>[2x]GPMKTEMKDDFAKLEEQFDAKLGIFALDTGTNRTVAYRPDERFAFASTIKALTVGVLLQQKSIEDLNQRITYTRDDLVNYNPITEKHVDTGMTLKELADASLRYSDNAAQNLILKQIGGPESLKKELRKIG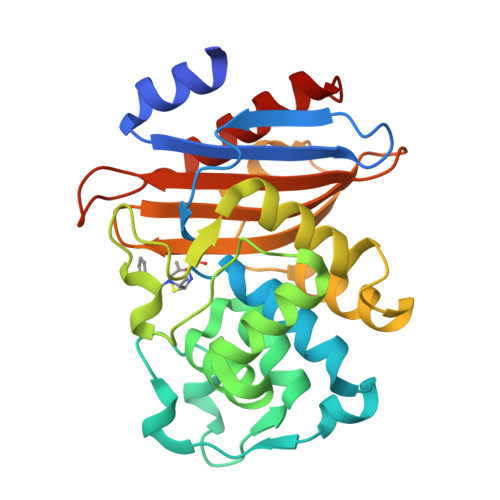DEVTNPERFYPELNEVNPGETQDTSTARALVTSLRAFALEDKLPSEKRELLIDWMKRNTTGDALIRAGVPDGWEVADKTGAASYGTRNDIAIIWPPKGDPVVLAVLSSRDKKDAKYDDKLIAEATKVVMKALNMNGK> MGVALGATRVIYPAGQKQEQLAVTNNDENSTYLIQSWVENADGVKDGRFIVTPPLFAMKGKKENTLRILDATNNQLPQDRE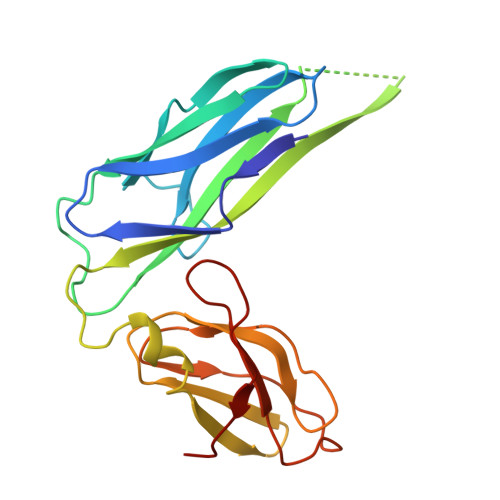SLFWMNVKAIPSMDKSKLTENTLQLAIISRIKLYYRPAKLALPPDQAAEKLRFRRSANSLTLINPTPYYLTVTELNAGTRVLENALVPPMGESTVKLPSDAGSNITYRTINDYGALTPKMTGVME> MGHHHHHHHHHHSSGENLYFQ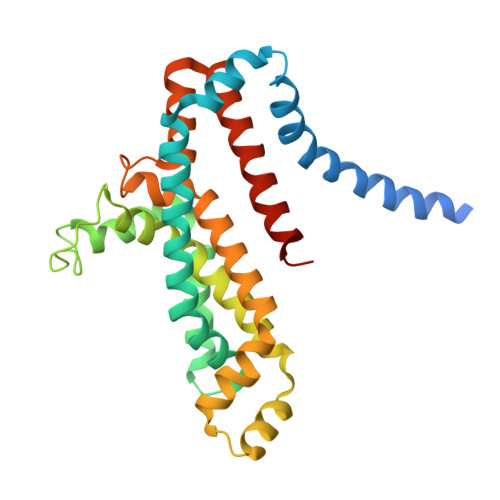GHMRLLFSALLALLSSIILLFVLLPVAATVTLQLFNFDEFLKAASDPAVWKVVLTTYYAALISTLIAVIFGTPLAYILARKSFPGKSVVEGIVDLPVVIPHTVAGIALLVVFGSSGLIGSFSPLKFVDALPGIVVAMLFVSVPIYINQAKEGFASVDVRLEHVARTLGSSPLRVFFTVSLPLSVRHIVAGAIMSWARGISEFGAVVVIAYYPMIAPTLIYERYLSEGLSAAMPVAAILILLSLAVFVALRIIVGREDVSEGQG> GLPTMLTPGSNQFLTSDDFQSPSAMPQFDVTPEMDIPGQVNNLMEIAEVDSVVPVNNTEGKVLSIESYQIPVQSNSTNGSQVFGFPLMPGASSVLNRTLLGEILNYYTHWSGSIKLTFMFCGSAMATGKFLLAYSPPGAGAPTTRKEAMLGTHVIWDVGLQSSCVLCIP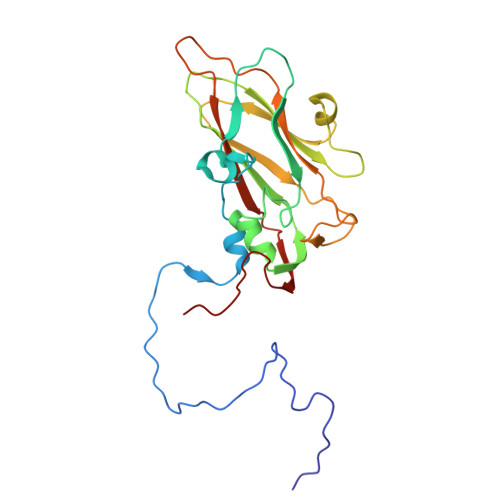WISQTHYRYVVVDEYTAGGYITCWYQTNIVVPADTQSDCKILCFVSACNDFSVRMLKDTPFIKQDNFYQ Biotin-dependent acetyl-CoA carboxylases (ACCs) are essential enzymes that catalyse the ATP-dependent carboxylation of acetyl-CoA to malonyl-CoA. Eukaryotic ACCs, instead, are multienzymes, which integrate all functional components into a single polypeptide chain of ∼2,300 amino acids2. In addition to the canonical ACC components, eukaryotic ACCs contain two non-catalytic regions, the large central domain (CD) and the BC–CT interaction domain (BT). Here we provide the structure of Saccharomyces cerevisiae (Sce) ACC CD, intermediate- and low-resolution structures of human (Hsa) ACC CD and larger fragments of fungal ACC from Chaetomium thermophilum (Cth).

Using molecular replacement based on fungal ACC CD and CT models, we obtained structures of a variant comprising CthCT and CDC1/CDC2 in two crystal forms at resolutions of 3.6 and 4.5 Å (CthCD-CTCter1/2), respectively, as well as of a CthCT linked to the entire CD at 7.2 Å resolution (CthCD-CT). In all these crystal structures, the CT domains build a canonical head-to-tail dimer29, with active sites formed by contributions from both protomers. The connection of CD and CT is provided by a 10-residue peptide stretch, which links the N terminus of CT to the irregular β-hairpin/β-strand extension of CDC2. The connecting region is remarkably similar in isolated CD and CthCD-CTCter structures, indicating inherent conformational stability. CD/CT contacts are only formed in direct vicinity of the covalent linkage and involve the β-hairpin extension of CDC2 as well as the loop between strands β2/β3 of the CT N-lobe, which contains a conserved RxxGxN motif. On the basis of an interface area of ∼600 Å2 and its edge-to-edge connection characteristics, the interface between CT and CD might be classified as conformationally variable. Indeed, the comparison of the positioning of eight instances of the C-terminal part of CD relative to CT in crystal structures determined here, reveals flexible interdomain linking. The CDC2/CT interface acts as a true hinge with observed rotation up to 16°, which results in a translocation of the distal end of CDC2 by 8 Å.

>[2x]GNLREVRYHDEERPYFIDWDFALRKSGANQTESSMHMQSVVPSSPATPVENDFKRIHSISDMTYLARRTRDEPIRKGVIVPCKDLLDAEEALSRALEVLPLAHKETKDKDRKQQPGIAADLAQRRRPGTPLRLEGIGELSAVVNVAVRDAEGKNDEEILALIKPWVQNSKADLLARRVRRLTFICGRNDGSYPSYYTFRGPDYAEDDSIRHIEPSLAFQLELGRLSKFKLTPVFTQNKNIHVYEAVGRGVETDRRYFTRAVVRPGRLRDEISTAEYLISEADRVVNDIFDALEIIGTNKTDLNHMFINFSHTFQVTADEVAESLQGFLDRFGPRGWRLRVHQVEIRINCMRSDNNDENDTMPLRVIITNTSGFVIQIELYEEKLSEKGEWVYYYVSGNAKIGSMHLLPVSTPYPTKNWLQPKRYKAHILGTQYVYDFPELFRQAIQNSWTEAVKKIPSLAAKQPAIGECIDYNELVLGDQDNLAEVSREPGMNSTGMVGWLINARTPEYPDGRKFIVVANDITFKIGSFGPKEDTFFFKCTELARKMGIPRIYLSANSGARLGLAEELMPHFNVAWNDPAKPEAGFKYLYLSDEAKRRFENEVITEEIVEDGEKRHKIITIVGAEEGLGVECLRGSGLIAGATSRAYNDIFTCTLVTCRSVGIGAYLVRLGQRAVQVEGQPIILTGAPALNSLLGREVYTSNLQLGGTQIMYRNGVSHLTAKDDFDGVTKIVQWLSFIPDQRNNPLPILSPSPDPWDRDVVYTPPYKQTYDVRWMIAGKEDEDGFQPGLFDKDSFVETLGGWARTVVVGRARLGGIPMGVIAVETRTIENITPADPANPDSIEQVTNEAGGVWYPNSAFKTAQAINDFNYGEQLPLMILANWRGFSGGQRDMYNEVLKYGSFIVDALTRFEKPIFIYIPPHGELRGGSWVVVDPTINPASMEMYADEEARGGVLEPEGIIPIKYKKDKQLETMARLDPVYRSLKKEMAKEGLSKEESDNIKKKMQQREELLLPIYHQICVQFADLHDRAGRMKAKGVIRQSLQWRQSRRFFYWRVRRRLIEDDILRRIEEAINPAGKRRHDPENTSLAASPETRSPHLVQLESWVGIPGFKTNDREVVEWYEQNQDRINEKLEKLKKESIADQMRELLRXXXXXXXXXXXX>MPENPAAEKMQV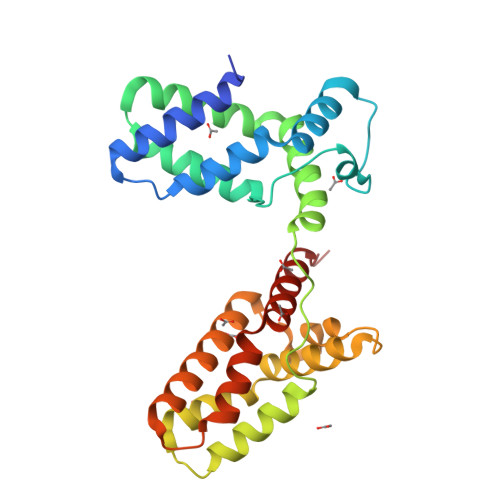LQVLDRLRGKLQEKGDTTQNEKLSAFYETLKSPLFNQILTLQQSIKQLKGQLSHIPLEVLFQGPVKILEIEDLFSSLKHIQHTLVDSQSQEDISLLLQLVQNKDFQNAFKIHNAITVHMNKASPPFPLISNAQDLAQEVQTVLKPVHHKEGQELTALLNTPHIQALLLAHDKVAEQEMGGGLEVLFQGPALVEPLGLERDVSRAVELLERLQRSGELPPQKLQALQRVLQSRFCSAIREVYEQLYDTLDITGS[4x]>MAHHHHHHMIRSDLQARHAEAFRALHTRPGAFIIPNPWDAGTARLLAMAGFEALATTSAGYAFSKGQPDNAIDRDAMLDHIADLVAAGGLPVSADLENGFGDAPGTVAETIRLAAEAGAVGGSIEDATGRADTPIYARDASVERIAAAVDAARALPFPFTLTARCENYLHGRRDLDDTIARLVAYRDAGADVLYAPGITDADEIAAVTRAVGAPVNVVMGLQGGLLSLDELAALGVKRVSVGGALARAALGAFLRAATEMRRDGTFTFTQAAVPGRD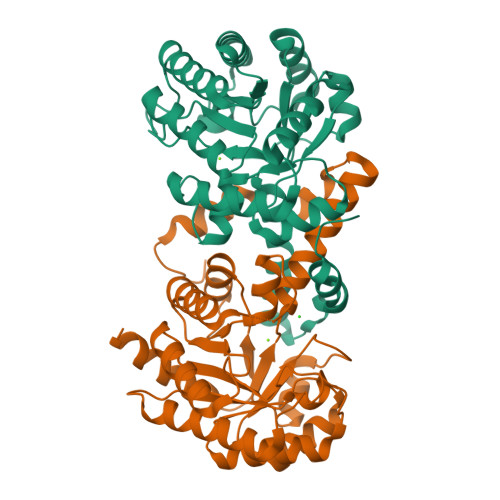INRWFAAPDNSPILFDE[2x]>[20x]GSHMLEGGVEVLSVVTGEDSITQIELYLNPRMGVNS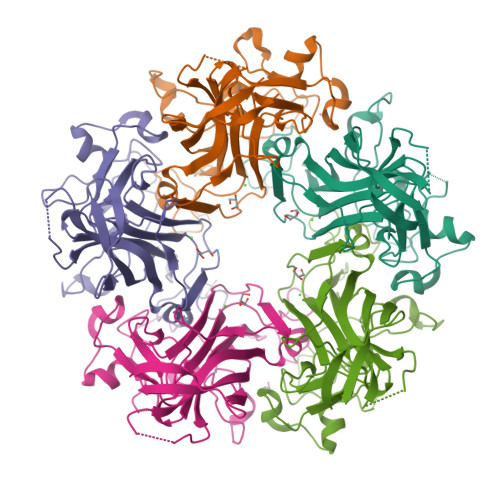PDLPTTSNWYTYTYDLQPKGSSPDQPIKENLPAYSVARVSLPMLNEDITCDTLQMWEAISVKTEVVGISSLINVHYWDMKRVHDYGAGIPVSGVNYHMFAIGGEPLDLQGLVLDYQTQYPKTTNGGPITIETVLGRKMTPKNQGLDPQAKAKLDKDGNYPIEVWCPDPSKNENSRYYGSIQTGSQTPTVLQFSNTLTTVLLDENGVGPLCKGDGLFISCADIVGFLFKTSGKMALHGLPRYFNVTLRKRWVKN> MQSPHAKYLRECLSLAEKSPPRPTNFRVGAILVSRKE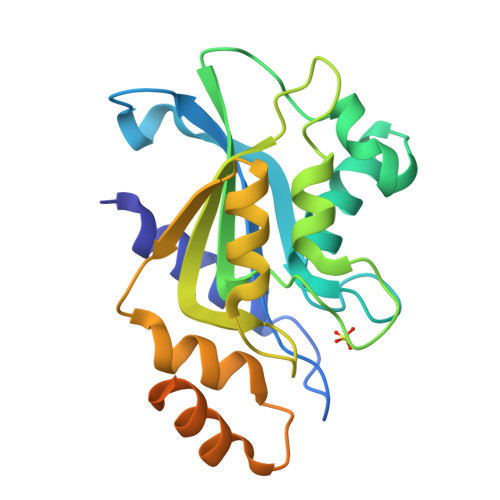GDYKTEDDRIVSTGYTMELAGNTHAEQCCLSNYAAVHSVPEDRVWEVLPSEPDRKLVMYVTMEPCGKRLSGNLPCVQRIIRTRQGDRKGIQKIYFGVKEPGTFVGGSEGCQMLTAAGIDWQVVNGLEREILEVAVAGHENREEEVKAALDTVETNIDDISDDERRRQQEAQRNPKKRMMEANLLGLEHHHHHH>[6x]PHMQPFDSGHDDLVHDVVYDFYGRHVATCSSDQHIKVFKLDKDTSNWELSDSWRAHDSSIVAIDWASPEYGRIIASASYDKTVKLWEEDPDQEECSGRRWNKLCTLNDSKGSLYSVKFAPAHLGLKLACLGNDGILRLYDALEPSDLRSWTLTSEMKVLSIPPANHLQSDFCLSWCPSRFSPEKLAVSALEQAIIYQRGKDGKLHVAAKLPGHKSLIRSISWAPSIGRWYQLIATGCKDGRIRIFKITEKLSPLASE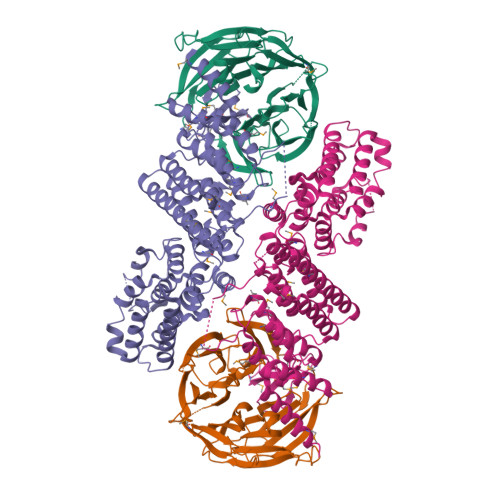ESLTNSNMFDNSADVDMDAQGRSDSNTEEKAELQSNLQVELLSEHDDHNGEVWSVSWNLTGTILSSAGDDGKVRLWKATYSNEFKCMSVITAQQ;>MTIDDSNRLLMDVDQFDFLDDGTAQLSNNKTDEEEQLYKRDPVSGAILVPMTVNDQPIEKNGDKMPLKFKLGPLSYQNMAFITAKDKYKLYPVRIPRLDTSKEFSAYVSGLFEIYRDLGDDRVFNVPTIGVVNSNFAKEHNATVNLAMEAILNELEVFIGRVKDQDGRVNRFYELEESLTVLNCLRTMYFILDGQDVEENRSEFIESLLNWINRSDGEPDEEYIEQVFSVKDSTAGKKVFETQYFWKLLNQLVLRGLLSQAIGCIERSDLLPYLSDTCAVSFDAVSDSIELLKQYPKDSSSTFREWKNLVLKLSQAFGSSATDISGELRDYIEDFLLVIGGNQRKILQYSRTWYESFCGFLLYYIPSLELSAEYLQMSLEANVVDITNDWEQPCVDIISGKIHSILPVMESLDSCTAAFTAMICEAKGLIENIFEGEKNSDDYSNEDNEMLEDLFSYRNGMASYMLNSFAFELCSLGDKELWPVAIGLIALSATGTRSAKKMVIAELLPHYPFVTNDDIEWMLSICVEWRLPEIAKEIYTTLGNQMLSAHNIIESIANFSRAGKYELVKS[6x]~{N}-[azanyl(azanylidene)methylidene]-5-fluoranyl-8-[2,4,6-tris(fluoranyl)phenyl]-3,4-dihydro-1~{H}-isoquinoline-2-carboxamide | C17 H14 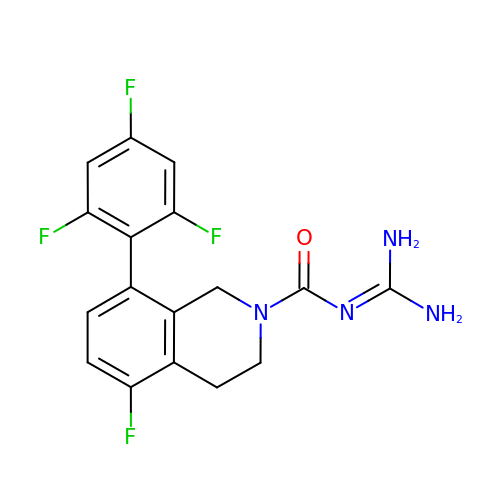F4 N4 O | YBJHLGWWZWMRCD-UHFFFAOYSA-N>GPGMKFKIDYELPLTSVAGKIRIKQRSTFNDYGLPVAPTKININVKHYVEWQIGYDMVAGKNDGNFIGANGKDKKLYELSDIIFQFFKHNIILKENLFGIKNFLENNEELIEDKMKINRTNFTQKQVAGINFLESYVSYPLLVYQFNNNEFLSEIIIKEKQRAIGVQGMLYFCFPVHLLKNINGERNFLNRSIESKEKGYLEISRNNINIFLEMLKIFGILSNNHRYNVLQIIEFILNSK[2x]

The most striking difference between R.PabI and R.CcoLI is that R.CcoLI cleaves the DNA backbone at medium temperatures, while the DNA backbone cleavage activity of R.PabI is very low at medium temperatures; R.PabI only hydrolyzes the N-glycosidic bond of the recognition sequence at medium temperatures. Both R.PabI and R.CcoLI are members of the HALFPIPE superfamily of restriction enzymes. Structural studies have identified that HALFPIPE superfamily proteins are not restriction endonucleases, but rather are restriction DNA glycosylases. However, at medium temperatures, R.PabI acts as a monofunctional DNA glycosylase, while R.CcoLI acts as a bifunctional DNA glycosylase. R.CcoLI is predicted to recognize a negatively charged dsDNA in the HALFPIPE region, similar to R.PabI.

The R.CcoLI structure was determined at a resolution of 2.35 Å using the crystal of the R.CcoLI(C189S-D225N) mutant. The final model contained one R.CcoLI dimer (chains A and B) in the asymmetric unit. R.CcoLI consists of five α-helices, fifteen β-strands and one 310 (η)-helix and forms the characteristic HALFPIPE structure using strands β3-β2-β5-β13-β12-β11. In this region of R.CcoLI, three catalytic residues of R.PabI, that is, Tyr68, His211 and Asp214, are conserved as Tyr52, His222 and Asp225, respectively. In the R.CcoLI structure, the insertion residues of R.CcoLI forms an antiparallel β-sheet (β6-β8-β7) adjacent to the active site. However, in the R.CcoLI structure, the side-chain orientation of Lys71 is flipped to the active site due to the insertion of the R.CcoLI specific antiparallel β-sheet. The model structure of the R.CcoLI-product DNA complex shows that the distance between the side-chain amine group of Lys71 and the C1′ carbon atom of cleaved deoxyadenosine is approximately 3 Å. In contrast, the results of the DNA glycosylase assay of the K71A-D225N mutant showed that the fraction of cleaved DNA was highly increased by NaOH treatment. This result indicated that the K71A-D225N mutant of R.CcoLI functions as a monofunctional DNA glycosylase and that the side-chain amine group of Lys71 is important for the DNA cleavage activity of R.CcoLI. In the R.CcoLI structure, this region shows relatively high temperature factors compared to the protein core region. Although the structure of R.CcoLI was determined in the absence of DNA, the R.CcoLI structure is most similar to the R.PabI structure in the sequence-nonspecific dsDNA-binding state.> MSLNDFLSSVLPVSEQFEYLSLQSIPLETHAVVTPNKDDKRVPKSTIKTQHFFSLFHQGKVFFSLEVYVYVTLWDEADAERLIFVSKADTNGYCNTRVSVRDITKIILEFILSIDPNYYLQKVKPAIGGSGFQQDLYLSFTCPREILTKICLFTRPASQYLFPDSSKNSKKHILNGEELMKWWGFILDRLLIECFQ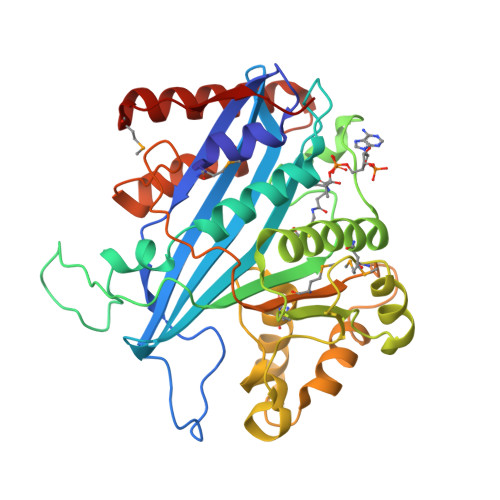NDTQAKLRIPGEDPARVRSYLRGMKYPLWQVGDIFTSKENSLAVYNIPLFPDDPKARFIHQLAEEDRLLKVSLSSFWIELQERQEFKLSVTSSVMGISGYSLATPSLFPSSADVIVPKSRKQFRAIKKYITGEEYDTEEGAIEAFTNIRDFLLLRMATNLQSLTGKRE>MSLIRMALAAVCALLFSITTMTPFVQASEITISGSTSVARIMDVLAEKYNQQHPETYVAVQGVGSTAGISLLKKGVADIAMTSRYLTESEAQNTLHTFTLAFDGLAIVVNQANPVTNLTREQLYGIYKGQITNWKQVGGNDQKIAVVTREASSGTRYSFESLMGLTKTVKDREVSDVAPTALVVNSNSMMKTLVNHNTQAVGFISIG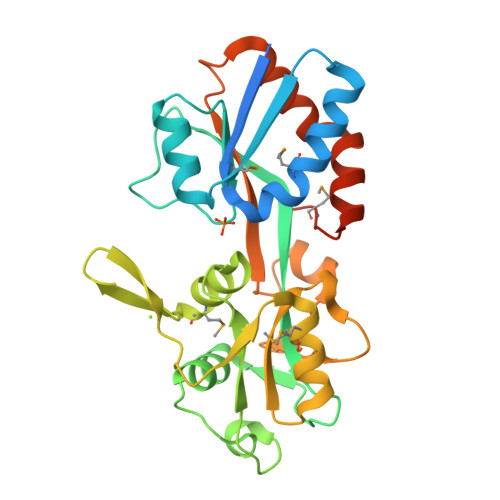SVDKSVKAIQFEKADPTSDNIAKHTYQLSRPFLILHYSDNADEQTKEFIAFLKSESAKKLIVEYGYIMPSDVEEGGSHHHHHH[8x]> MRGSHHHHHHGSMVAPTSNPGVPDELDGVPAVVDCDVHAVLPSPHSLIPYLDEYWADQLVAQLAPTYEPNYHPRGSAIAQHSDASVDENGRAATTAENLVKDVFADGFTDFAVVNCLYGVQQIHQPRREMAHARALNHWIANEWLDKDDRLRASIVVPQGSPRAAAEEIDFWSGDKRFVQVLLLGQSELLYGREINWPIWEAAEAAGLPVTLHIGGVFRQAPTS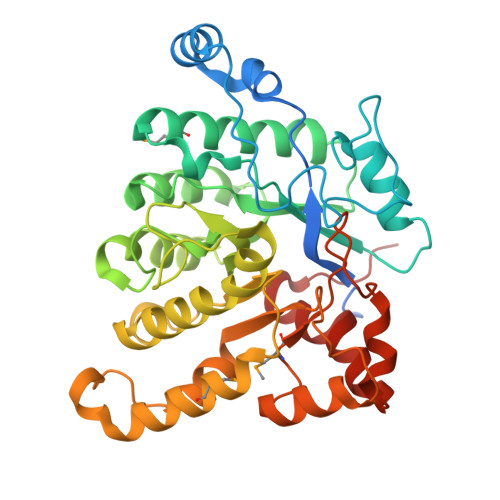VGWPASHLEWYVGQQSNIEAQLNSIISEGILQKFPKTKILLSELGFNWLPPFMWKFDKLWKSYRPDIPWVQESPLELIREHVRVTTSPSDGAEEAGRLDSIVDRLGSDRMLVYSSDYPHKHHSGPRDIENGTHSPELLDRIYRRNAFDLYNLVVPSPGKVG> MELIKGQALFLELDKKDFLSLKNNDKNIPTFAHPKNQEKILAIFSLPYKNPPQNTKLIAFYKDKKEEIFIKTLEGNYKSEKLQVENKKIFPPKTIQERIAKELKEANAIYSSYTPKALFNGAFNIPLNSFITSDFGKARTFNEKVASYHSGTDFRAATGTPIYAANSGVVKIAKDRYFAGNSVVIDHGFGIYSQYYHLSKIDVKVGQKIKKGELIGLSGASGRVSGPALHFGILAGGKQVDPLDFVSKFNAIFQLEHHHHHH

We have described herein the reactions and the structure of Pgp3, a Csd protein of C. jejuni. This enzyme turns over the cell-wall peptidoglycan by both the d,d-endopeptidase and d,d-carboxypeptidase activities, as documented by mass spectrometric characterization of the requisite reactions with synthetic cell-wall fragments. The Pgp3 monomer is structurally divided into four regions: the N-terminal domain (NTD, residues 21–95), a flexible linker (residues 96–147), the LytM domain (residues 148–259), and the C-terminal helix (residues 260–273). The Pgp3 LytM domain contains a highly conserved tetrahedral Zn2+-ion-binding motif (H168xxxD172 and HxH249).

We decided to mutate His216 and His247 individually to alanine in order to abrogate the binding of tartrate or citrate at the active site and impair catalysis too. Indeed, when we solved the crystal structure of the H247A variant, it showed the absence of citrate or tartrate electron densities within the active site and the protein only assumed the open conformation, which was fortuitous for efforts toward solving the structure of the enzyme complexes with substrate analogs. In the uncomplexed H247A variant, two water molecules (Wat-1 and Wat-2) occupy the active site. Because Wat-1 and Wat-2 were essentially equidistant from Zn2+ (2.9 Å and 2.7 Å, respectively), we could not establish which should be the hydrolytic-water molecule. However, the crystal structure of the H247A variant in complex with the substrate clearly showed that Wat-2 was replaced by the incoming substrates, concluding that Wat-1 is the hydrolytic water that attacks the scissile carbonyl group of substrates. The distance between Wat-1 and Zn2+ decreases from 2.7 Å in the uncomplexed H247A variant to 2.6 Å in the complexed one.> KVFERCELARTLKRLGMDGYRGISLANWMCLAKWESGYNTRATNYNAGDRSTDY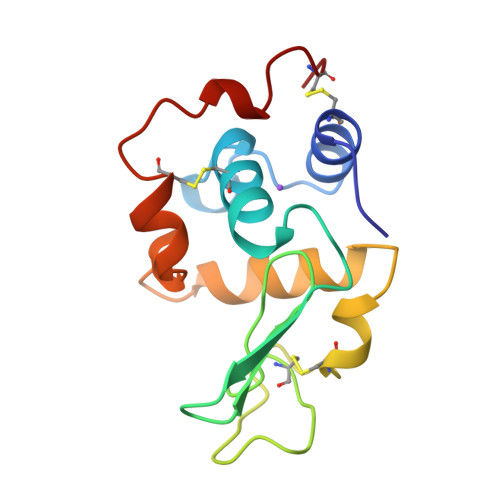GIFQINSRYWCNDGKTPGAVNAAHLSCSALLQDNVADAVAAAKRVVRDPQGIRAWVAWRNRCQNRDVRQYVQGCGV> GSMAKVQVNNVVVLDNPSPFYNPFQFEITFECIEDLSEDLEWKIIYVG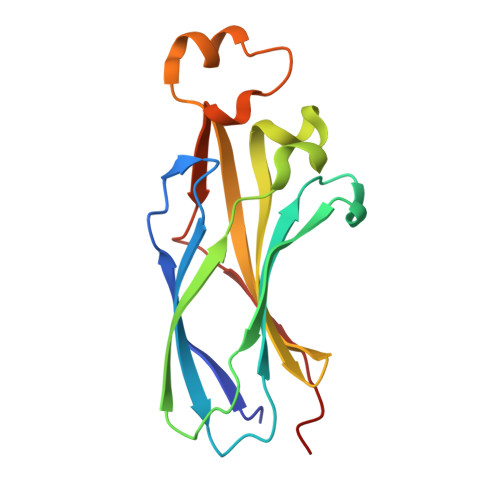SAESEEYDQVLDSVLVGPVPAGRHMFVFQADAPNPGLIPDADAVGVTVVLITCTYRGQEFIRVGYYVNNEYTETELRENPPVKPDFSKLQRNILASNPRVTRFHINWED>SQANLMRLKSDLFNRSPMYPGPTKDDPLTVTLGFTLQDIVKVDSSTNEVDLVYYEQQRWKLNSLMWDPNEYGNITDFRTSAADIWTPDITAYSSTRPVQVLSPQIAVVTHDGSVMFIPAQRLSFMCDPTGVDSEEGVTCAVKFGSWVYSGFEIDLKTDTDQVDLSSYYASSKYEILSATQTRQVQHYSCCPEPYIDVNLVVKFRERRAGNGFFRNLFDHHHHHH[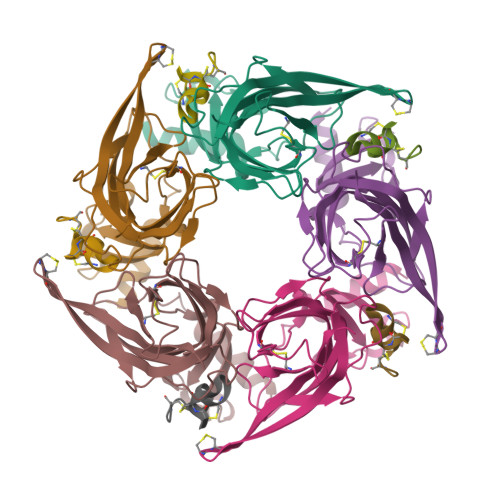5x];>[5x]GCCSHPACNVDHPEICX> MEWSQIFHDITTKHDFKAMHDFLEKEYSTAIVYPDRENIYQAFDLTPFENIKVVILGQDPYHGPNQAHGLAFSVQPNAKFPPSLRNMYKELADDIGCVRQTPHLQDWAREGVLLLNTVLTVR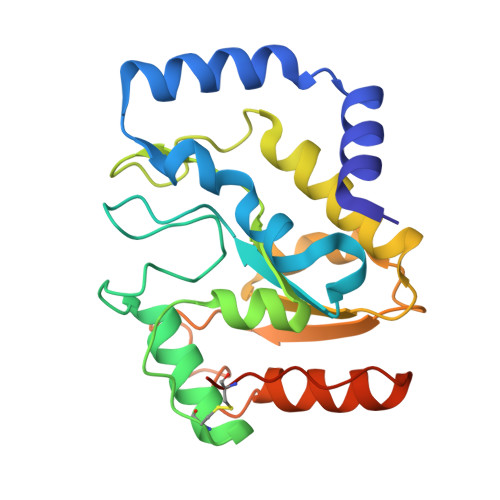QGEANSHRDIGWETFTDEIIKAVSDYKEHVVFILWGKPAQQKIKLIDTSKHCIIKSVHPSPLSAYRGFFGSKPYSKANTYLESVGKSPINWCESEALEHHHHHH> MQDNSRYTHFLTQHYDAKPQGRDDRYCESIMRRRGLTSPCKDINTFIHGNKRSIRAICENKNGNPHRENLRISKSSFQVTTCKLHGGSPWPPCQYRATAGFRNVVVACENGLPVHLDQSIFRRP

Angiogenin (ANG), a 14-kDa basic protein is an angiogenic ribonuclease and member of the bovine pancreatic ribonuclease (RNase A) family (also known as RNase 5). Like RNase A, ANG cleaves preferentially on the 3′ side of pyrimidines and follows a transphosphorylation/hydrolysis mechanism. In addition, the crystal structure of human ANG has revealed that it has an RNase A fold and the catalytic triad (residues H13, K40 and H114) is conserved. The enzymatic activity of ANG is several orders of magnitude lower than that of RNase A towards conventional RNase substrates, but essential for its angiogenic effect.

K54 does not participate or belong to any of the known catalytic sub-sites of ANG6. The variant K54R retains ~49% of enzyme activity. In this PD variant structure this residue is exposed on the surface of the molecule. Also, in the variant structure the Arg side chain makes a water mediated interaction with R51.Type IV-A CRISPR-Cas systems diverge from this general mechanism, using a nuclease-independent interference pathway to suppress gene expression for gene regulation and plasmid competition. Here, we present several cryo-EM structures of two evolutionary distant type IV-A1 and type IV-A3 complexes (from Pseudomonas oleovorans and Klebsiella pneumoniae, respectively) bound to cognate DNA targets with and without DinG. The structures reveal multisubunit DNA-surveillance complexes that intimately recognize their DNA-targets to form an R-loop structure. Our results support a model in which DNA-binding is achieved analogously to type I Cascade, while recruitment of DinG differs mechanistically, even in closely related subtypes.

Cryo-EM grid optimization and exhaustive data collection yielded a sufficient amount of particles to reconstruct three structures of the DinG-bound type IV-A3 effector complex, with DinG resolved at ~3 Å to ~7 Å in three distinct states (states I–III). Similar to the type IV-A1 structure, type IV-A3 DinG is recruited to the NTS at the belly side of the complex. But unlike type IV-A1 DinG, type IV-A3 DinG contacts the palm domains of Cas5, Cas7.1 and Cas7.2 through HD2 domain α-helices 22–25, and interacts with the thumb-domain α-helices 8 and 9 of Cas7.3. Moreover, arch domain α-helices 14 and 15 are near Cas7’s WL motif, and DinG inserts its C-terminal tail into a cleft formed between Cas8’s CTD and the palm of Cas5, thereby anchoring the HD2-domain poised for NTS recruitment. Collectively, these results suggest that the interface between DinG HD2 α-helices (α22, α23) and Cas7’s palm primarily determines DinG recruitment. We next compared the three type IV-A3 DinG states, based on a structural alignment of the complexes. This revealed that the Cas8 and Cas5 contacting C-terminus, and Cas7 palm binding segments of α-helices 21 and 22 of DinG, do not rearrange between the states. Thus, the C-terminus and α-helices 21 and 22 appear to anchor DinG to the complex. The arch domain becomes stabilized in state I, as corroborated by the absence and presence of cryo-EM density in states II and I, respectively. Additionally, the arch domain rearranges and becomes stabilized in state I, as evidenced by the less pronounced cryo-EM density in state III. Examination of the cryo-EM map also revealed low local resolutions (4–7 Å) for the vFeS domain and NTS exiting the HD2 in all states.

>[6x]MRTLNFNGKISTLEPLTVTVKNAVSTSGHRLPRNGGFNAAPYFPGTSIRGTLRHAAHKVIVDRVGLNADGKSPFDLAEHFMLAQGVDINGEAETFAPGEINAGAELRSKNPLISLFGRWGLSGKVGIGNAIPDGDNQWGMFGGGARSIMFQRDESLMEFLETDQVDRLERLLEEQAEASVDISQIKTEQDALKKAMKSADKDTKAELQIKVRELDEKIQARKDQKQESRESIRRPIDPYEAFITGAELSHRMSIKNATDEEAGLFISALIRFAAEPRFGGHANHNCGLVEAHWTVTTWKPGELVPVTLGEIVITPNGVEITGDELFAMVKAFNENQSFDFTARGHHHHHH;> MLNFKPYRVIMSSLTPVVISGIAPSLDGILYEALSQAIPSNEPGVVLARLKEILLFNDELGVFHASSLRFGITPEQGIGATTSMRCDYLSPEKLSTAMFSPRTRRGLFTRVLLTGGPTKRRMTTRPAYSAPYLTFDFVGSSEAVEILLNHAHVGVGYDYFSAANGEFNNVTILPLDIDTSISNEGMALRPVPVNSGLNGIKGVSPLIPPYFVGEKLNIVHPAPVRTQLISSLLRG;> MNHPVESVYSALTSILLPYMGEPVPVQRNCSCCGRAPSEFDGVGFELVNAYRERVVHCRPCQTFFVSAPELMGVENPKKPTTGQKFGMWSGVGAVINVEDNSSVLLAPQGVVNKLPEHFFDHVEVITATSGQHLEYLFNTELKFPLIYIQNFGVKTYELVRSLRVSLSADAIYTCADQLLTRQNEVLYMLDLKKAKELHQEIKNYSKKEMDIFIRTVTLLAYSRITPEAASNEFKKNNLIPLLLLLPTDPHQRLSILHLLKKV;> MNTSAVFESAGLSLRKVQQDYIEAAAGALTQDHKVALISAETGVGKTLGYLVPALLILLKNPEAKFVIATNSHALMHQIFRSDRPLLEQIAEQCGIKVTFSRLMGKANYVSLEKVRGLLLMDEFTDLDTVKVLEKLANWSKPLVEFEEEYGELPAQITPEMVTYSIWDDIQDIDDIRLNALSANFIVTTHAMVMVDCMCNHRILGDKENMYLIIDEADIFVDMLEVWKQRRFNLRELTSAFNEHIPRNGVHVIDQLMNDVTSIAGDLHFCSTPAAVALFDNSFNALSKVGREIKNEAARKAFFDCIYSWEMLGLSGGQKGVGVSNKRREPALIAVNPFIGMNVGRYCTQWRSALLTSATLSITSTPETGMEWLCKALGLTSDTISIRKIFSPDVYGSMKLTIAGADFPKVFNDPKEQIFSGQWLKAVVEQLSCIQGPALVLTASHYETRMIANQLGEVSQPVYIQKAGQALSEIIKQYQEKPGILISAGASVGVSPRGENGEQIFQDLIITRIPFLPPDRMKAESLYGYLKERGYSRTFEAVNRNIYLENLRKVIRKAKQSVGRGIRSENDTVRIIILDPRFPEPTDLSSKHRSLEHIIPVRFRREYRSCEILSPAYFEEDIQC>MTKAVHTKHAPAAIGPYSQGIIVNNMFYSSGQIPLTPSGEMVNGDIKEQTHQVFSNLKAVLEEAGASFETVVKATVFIADMEQFAEVNEVYGQYFDTHKPARFCVEVARLPKDALVEIEV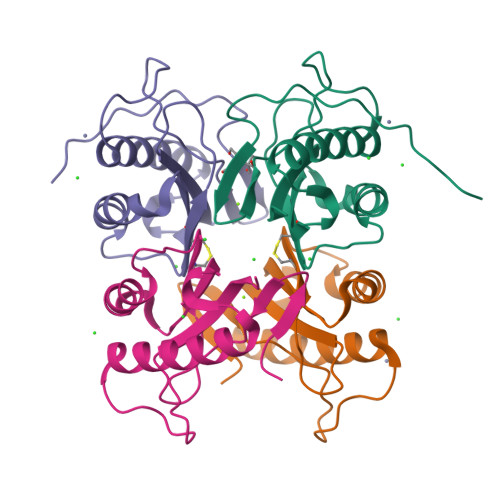IALVK[4x]> MGSDKIHHHHHHVRVLAIRHVEIEDLGMMEDIFREKNWSFDYLDTPKGEKLERPLEEYSLVVLLGGYMGAYEEEKYPFLKYEFQLIEEILKKEIPFLGICLGSQMLAKVLGASVYRGKNGEEIGWYFVEKVSDNKFFREFPDRLRVFQWHGDTFDLPRRATRVFTS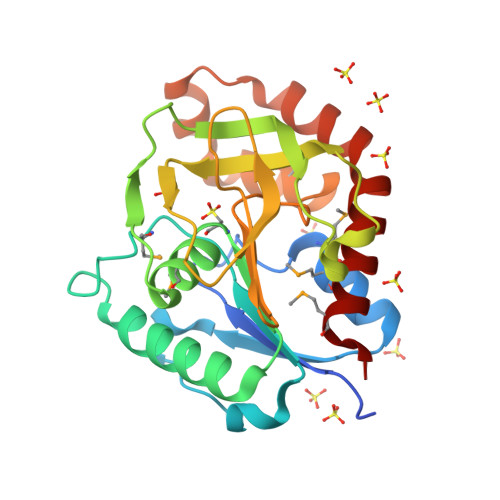EKYENQGFVYGKAVGLQFHIEVGARTMKRWIEAYKDELEKKKIDPRLLLETAEREEKVLKGLLRSLLERMVES3,3'-(benzo[1,2-d:5,4-d']bis[1,3]thiazole-2,6-diyl)dipropanoic acid | C14 H12 N2 O4 S2 | 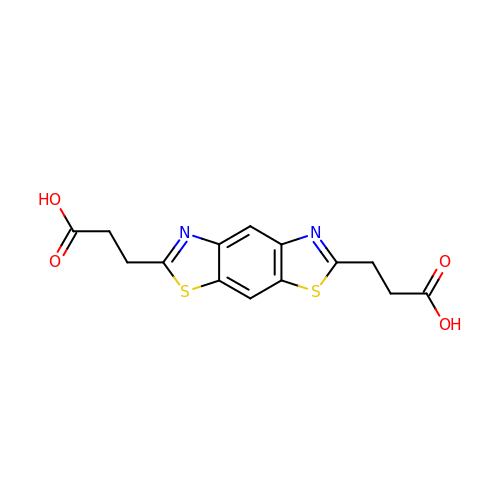RNLHVOCFLIRTNO-UHFFFAOYSA-N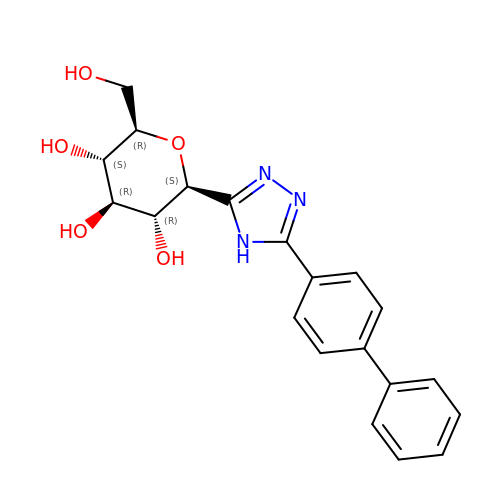(2~{R},3~{S},4~{R},5~{R},6~{S})-2-(hydroxymethyl)-6-[5-(4-phenylphenyl)-4~{H}-1,2,4-triazol-3-yl]oxane-3,4,5-triol | C20 H21 N3 O5 | NIARDQNUDKGRGO-UYTYNIKBSA-N>[4x]QTGGSFFEPFNSYNSGTWEKADGYSNGGVFNCTWRANNVNFTNDGKLKLGLTSSAYNKFDCAEYRSTNIYGYGLYEVSMKPAKNTGIVSSFFTYTGPAHGTQWDQIDIQFLGKDTTKV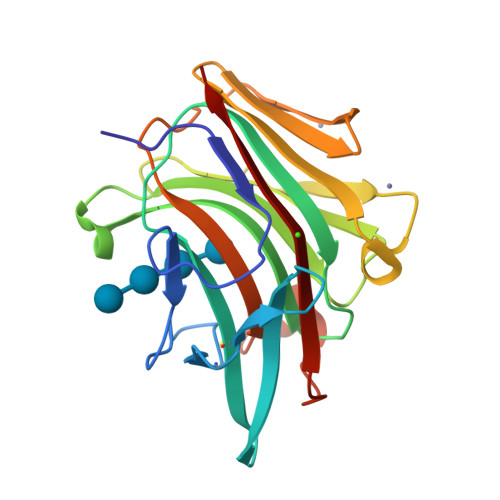QFNYYTNGVGGHEKVISLGFDASKGFHTYAFDWQPGYIKWYVDGVLKHTATANIPSTPGKIMMNLWNGTGVDDWLGSYNGANPLYAEYDWVKYTSN> ASNLKTEQAILTPPPMVPPAINRDHSAKVVINLETREQVGRIADGVEYVFWSFGETVPGSFIRVREGDEIEFNLSNHPSSKMPHNIDLHAVTGPGGGAESSFTAPGHTSTFNFKALNPGLYIYHCATAPVGMHIANGMYGLILVEPKEGLAPVDREYYLVQGDFYTKGEFGEAGLQPFDMAKAIDEDADYVVFNGSVGSTTDENSLTAKVGETVRLYIGNGGPNLVSSFHVIGEIFDTVYVEGG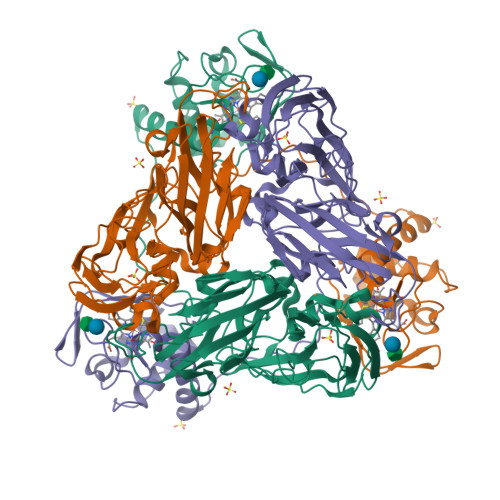SLKNHNVQTTLIPAGGAAIVEFKVEVPGTFILVDHSIFRAFNKGALAMLKVEGPDDHSIFTGKTAENVYLPEGSAIQSLDNTFTKITANNKDEQIRFGQRVYEANCMACHQANGEGIPGAFPPLAKSDYLNNNPLLGVNAIIKGLSGPIKVNNVNYNGVMPAMNLNDEDIANVITFVLNNWDNAGGKVSAEQVAKQRK> GUACGAAGGAAGGUUUGGUAUGGGGUAGUU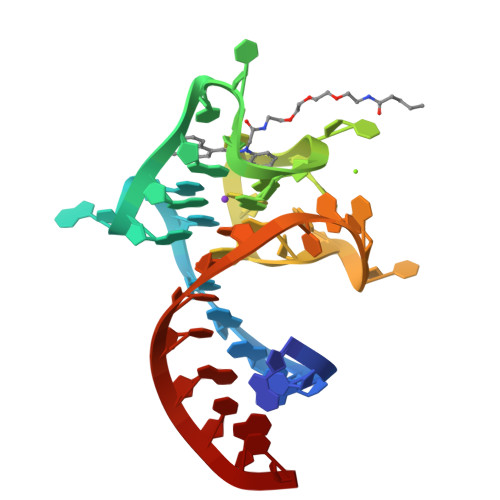GUCGUAC>[3x]GAMDPGEETINSTQNKTRTKTTRPKAVYLWTVSDVLKWYRRHCGEYTQYEQLFAQHDITGRALLRITDSSLQRMGVTDNRDREAIWREIVKQRLKTDIMEIRDM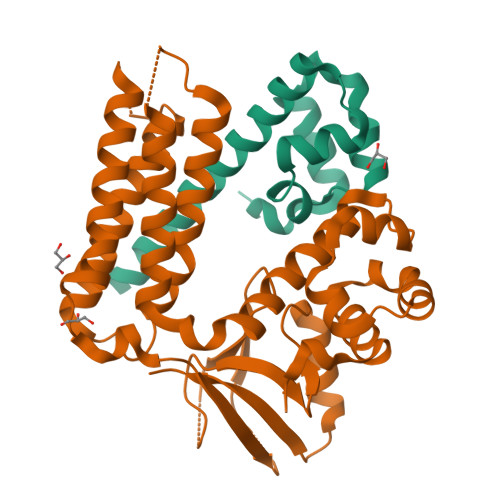ERLNIY;>GAMDPMAYINIAEWTPDQVTDWIKGLDESMKGYLYEFSKQEIGGRALLNIRPYELENLGMLRIGHQEIVLEAVENLRNFHYHLKNDNLQFMALHVATAAKNLHRELARNHAESTKIDTRILHDITRTIATLKPLVGSLERTPFRKQEMYREYCGNVLKCGLELATIAHRDRFALQPVPAIRQSAERLENLANFVIQDISDPMVLQPASLNLVTLKKRESELGFNIESSYNGIHRVTDIKYNSPAHNSGKIEDGDEIVQINYQTVVGWQHRTVLEHLREALPDVVLTVKKRPKHTKMFGQIYMQPYRLPSKKRNMAARWAAQMPSPRAAFLTLDTE[3x]>MAKKTSSKGKLPPGPFPLPIIGNLFQLELKNIPKSFTRLAQRFGPVFTLYVGSQRMVVMHGYKAVKEALLDYKDEFSGRGDLPAFHAHRDRGIIFNNGPTWKDIRRFSLTTLRNYGMGKQGNESRIQREAHFLLEALRKTQGQPFDPTFLIGCAPCNVIADILFRKHFDYNDEKFLRLMYLFNENFHLLSTPWLQLYNNFPSFLHYLPGSHRKVIKNVAEVKEYVSERVKEHHQSLDPNCPRDLTDCLLVEMEKEKHSAERLYTMDGITVTVADLFFAGTETTSTTLRYGLLILMKYPEIEEKLHEEIDRVIGPSRIPAIKDRQEMPY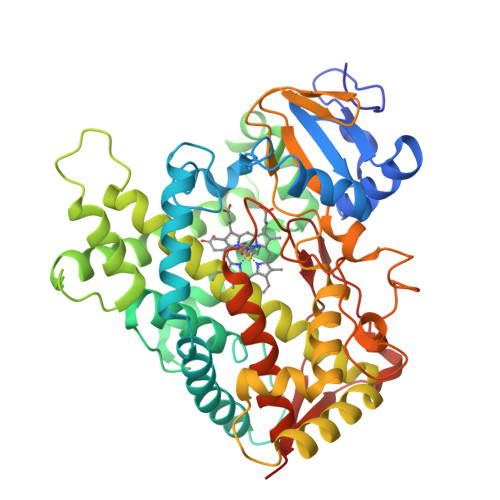MDAVVHEIQRFITLVPSNLPHEATRDTIFRGYLIPKGTVVVPTLDSVLYDNQEFPDPEKFKPEHFLNENGKFKYSDYFKPFSTGKRVCAGEGLARMELFLLLCAILQHFNLKPLVDPKDIDLSPIHIGFGCIPPRYKLCVIPRSHHHH[2x]> MGSSHHHHHHSQDMEAAIEFDEIVKKLLNIYINDICTTGEKRLLNNYEKSILDRIYKSCEYIKKNYELDFNSMYNQININNITTSDIKSKIIEALLIDSRPSVKLATLSFISLIAEKWGEKNRAKIMEILSNEIVEKISNNGKDFIDFIDRDDDDIVDDYVL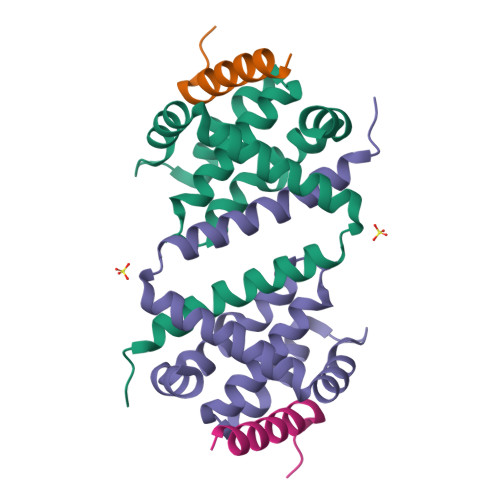ITNYLK;> PSSTMGQVGRQLAIIGDDINRRYDSE>[6x]EKKPYIISNVGMTLDGKLATINNDSRISCEEDLIRVHKIRANVDGIMVGIGTVLKDDPR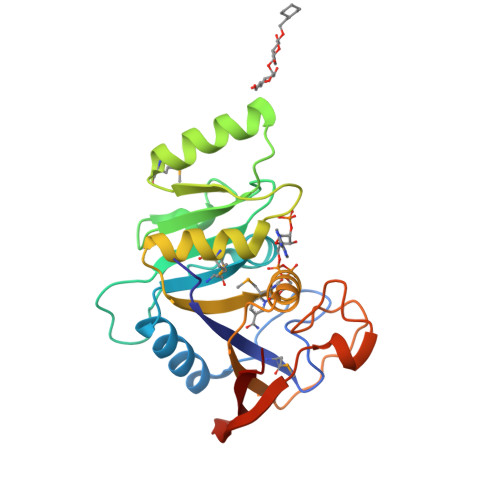LTVHKIKSDRNPVRIVVDSKLRVPLNARVLNKDAKTIIATTEDTNEEKEKKIKILEDMGVEVVKCGRGKVDLKKLMDILYDKGIKSILLEGGGTLNWGMFKEGLVDEVSVYIAPKIFGGKEAPTYVDGEGFKTVDECVKLELKNFYRLGEGIVLEFKVKK A glucosylglycerate hydrolase (GgH) identified in M. hassiacum and found to be highly conserved among rapidly growing mycobacteria is likely to be responsible for the rapid mobilization of GG accumulated during nitrogen starvation by hydrolysing it to glucose and glycerate. The MhGgH monomer displays an (α/α)6-barrel domain typical of glycoside hydrolase family 63 (GH63), to which MhGgH belongs. While the active site of GH63 members acting on larger substrates is located in an open, solvent-accessible cleft, those of MhGgH and of MgH from T. thermophilus are covered by a cap domain (subdivided into A′- and B′-regions) with constrained access through a narrow negatively charged tunnel. The crystallographic structure of MhGgH revealed a homotetrameric architecture, which is compatible with the oligomeric organization of the enzyme in solution as assessed by SAXS.

To avoid substrate hydrolysis during crystallization or soaking, three catalytically inactive variants of MhGgH were produced. Two putative catalytic residues (Asp182 and Glu419) and one substrate-interacting residue (Asp43) were identified and replaced by alanine to produce the D43A, D182A and E419A variants. The thermal stability of the D182A and E419A variants was comparable to that of wild-type MhGgH, while that of the D43A variant was slightly lowered (3°C) [Fig. 2(d)]. There is residual electron density compatible with presence of the substrates in the structures of the D182A and E419A variants, but not in that of the D43A variant, independent of the soaking time, highlighting the contribution of Asp43 to substrate binding.

>[2x]GAMPHDPSFTPTQLAARAAYLLRGNDLGTMTTAAPLLYPHMWSWAAAFVAIGLAPLSVERAVVELDTLLSAQWRNGMIPHIVFANGVDGYFPGPARWATATLADNAPRNRLTSGITQPPVHAIAVQRILEHARTRGRSTRAVAEAFLDRRWGDLMRWHRWLAECRDRNERGRITLYHGWESGMDNSPRWDSAYANVVPGKLPEYQRADNVIITDPSQRPSDGEYDRYLWLLEEMKAVRYDDERLPSVMSFQVEDVFFSAIFSVACQVLAEIGEDYKRPHADVKDLYLWAERFRAGVVETTDQRTGAARDFDVLAEKWLVTETAAQFAPLLCGGLPHDRERALLKLLEGPRFCGHPDLKYGLIPSTSPVSRDFRPREYWRGPVWPVLTWLFSWCFARRGWAERARLLRQEGLRQASDGSFAEYYEPFTGEPLGSMQQSWTAAAVLDWLG>[2x]MRSKRFEALAKRPVNQDGFVKEWIEEGFIAMESPNDPKPSIKIVNGAVTELDGKPVSDFDLIDHFIARYGINLNRAEEVMAMDSVKLANMLCDPNVKRSEIVPLTTAMTPAKIVEVVSHMNVVEMMMAMQKMRARRTPSQQAHVTNVKDNPVQIAADAAEGAWRGFDEQETTVAVARYAPFNAIALLVGSQVGRPGVLTQCSLEEATELKLGMLGHTCYAETISVYGTEPVFTDGDDTPWSKGFLASSYASRGLKMRFTSGSGSEVQMGYAEGKSMLYLEARCIYITKAAGVQGLQNGSVSCIGVPSAVPSGIRAVLAENLICSSLDLECASSND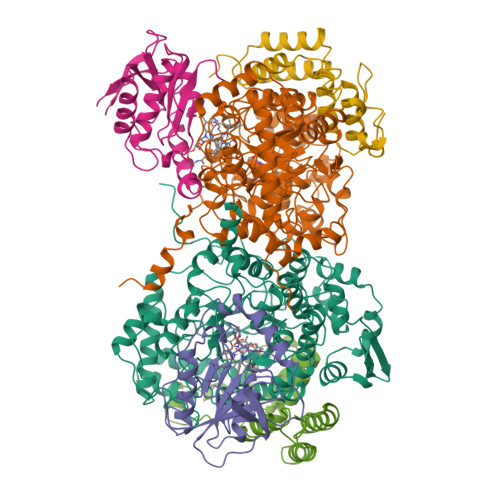QTFTHSDMRRTARLLMQFLPGTDFISSGYSAVPNYDNMFAGSNEDAEDFDDYNVIQRDLKVDGGLRPVREEDVIAIRNKAARALQAVFAGMGLPPITDEEVEAATYAHGSKDMPERNIVEDIKFAQEIINKNRNGLEVVKALAQGGFTDVAQDMLNIQKAKLTGDYLHTSAIIVGDGQVLSAVNDVNDYAGPATGYRLQGERWEEIKNIPGALDPNEID;>[2x]MEINEKLLRQIIEDVLSEMKGSDKPVSFNAPAASAAPQATPPAGDGFLTEVGEARQGTQQDEVIIAVGPAFGLAQTVNIVGIPHKSILREVIAGIEEEGIKARVIRCFKSSDVAFVAVEGNRLSGSGISIGIQSKGTTVIHQQGLPPLSNLELFPQAPLLTLETYRQIGKNAARYAKRESPQPVPTLNDQMARPKYQAKSAILHIKETKYVVTGKNPQELRVAL;>[2x]MNTDAIESMVRDVLSRMNSLQGEAPAAAPAAGGASRSARVSDYPLANKHPEWVKTATNKTLDDFTLENVLSNKVTAQDMRITPETLRLQASIAKDAGRDRLAMNFERAAELTAVPDDRILEIYNALRPYRSTKEELLAIADDLESRYQAKICAAFVREAATLYVERKKLKGDD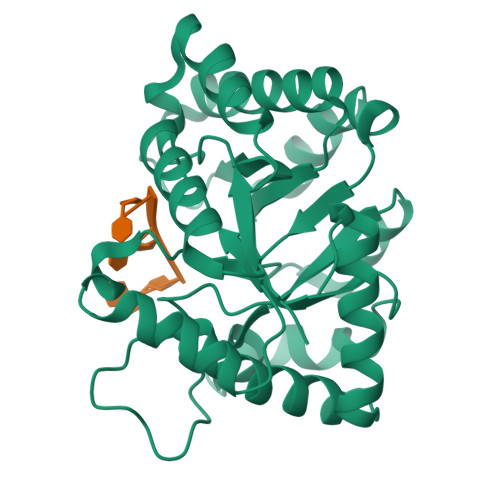> MFDIGVNLTSSQFAKDRDDVVACAFDAGVNGLLITGTNLRESQQAQKLARQYSSCWSTAGVHPHDSSQWQAATEEAIIELAAQPEVVAIGECGLDFNRNFSTPEEQERAFVAQLRIAADLNMPVFMHCRDAHERFMTLLEPWLDKLPGAVLHCFTGTREEMQACVAHGIYIGITGWVCDERRGLELRELLPLIPAEKLLIETDAPYLLPRDLTPKPSSRRNEPAHLPHILQRIAHWRGEDAAWLAATTDANVKTLFGIAF>[2x]SNAMHYQPKQDLLQNRIILVTGASDGIGREAALTYARYGATVILLGRN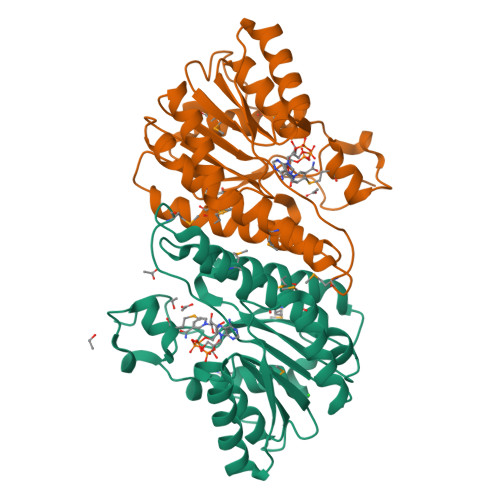EEKLRRVAQHIADEQHVQPQWFTLDLLTCTAEECRQVADRIAAHYPRLDGVLHNAGLLGEIGPMSEQDPQIWQDVMQVNVNATFMLTQALLPLLLKSDAGSLVFTSSSVGRQGRANWGAYATSKFATEGMMQVLADEYQNRSLRVNCINPGGTRTSMRASAFPTEDPQKLKTPADIMPLYLWLMGDDSRRKTGMTFDAQPGRKPGIAQ>[3x]GAMAMSDLPIEFTELVDLMSLGISPQFLDFRSTTFESDHFVTVRETKDGTNSVAIVDLAKGNEVTRKNMGGDSAIMHPSQMVISVRANGTIVQIFNLETKSKLKSFTLDEPVIFWRWLSETTLGFVTARSILTSNVFDGNVNAKPQLLTLRHANLNNTQIINFVANKNLDWFAVVGILQENGRIAGRIQLFSKQRNISQAIDGHVAIFTNILLEGNGSTPVQVFVTGNRNATTGAGELRIIEIDHDASLPSQYQKETTDIFFPPDATNDFPIAVQVSEKYGIIYLLTKYGFIHLYELETGTNLFVNRITAESVFTAAPYNHENGIACINKKGQVLAVEISTSQIVPYILNKLSNVALALIVATRGGLPGADDL;>[9x]GVSLIDL

The protein that gives the process its name, Clathrin, is a triskelion composed of three heavy chains (Clathrin Heavy Chain, Chc) that provide the structural backbone of the lattice, further stabilized and regulated by three light chains (Clathrin Light Chain, Clc). The proximal domain specifically interacts with Clcs, whereas, the N-terminal domain (NTD) of Chc, which adopts a WD40 beta-propeller structure, is pivotal for interactions with various adaptor proteins (APs). To investigate the existence of binding sites present in Clathrin NTD, we crystallized the N-terminal domain of Chc with different peptides derived from adaptor proteins containing CBMs. All our structures show that each peptide binds to three different binding pockets (Clathrin, Arrestin and W-box).

Crystal structure of Chc-NTD (displayed as a grey cartoon) bound to CBMs from Ent1 (1.75 Å, red), Ent2 (1.74 Å, yellow), Ent5 (Ent5.1 LIDL motif, 2.01 Å, green), Apl2.1 (Apl2.1 LLDLF motif, 2.75 Å, blue) and Yap1801 (1.95 Å, grey). Zoom: individual Chc-NTD boxes with Ent2 CBM-containing peptide. For the Ent1 and Ent2 complexes, a water molecule bridges the interaction between the carbonyl oxygen at the motif’s +3 position and N64. Water-mediated interactions are also observed in the W-box between the NTD backbone (L24, D25 and V309) and the peptide at position +3, for both Ent1 and Ent2. Residue K284 within the W-box establishes salt bridges with the carboxy-terminal of Ent1, Ent2 and Yap1801. For the Chc-mScarlet/Ent2-mNeonGreen pair, mutation of the Arrestin box showed a significant decrease in FRET efficiency (9.02% for WT vs. 6.7% Arr), while the W and Cla mutants did not show significant changes. Ent2’s main target site appears to be the Arrestin box as shown in our FRET in vivo experiments. Mutation of the Clathrin box showed a reduction of almost seven-fold in the binding affinity to Ent1 (KDApp WT ≅ 138 µM vs. KDApp Cla ≅ 968 µM), while Ent2 exhibits a three-fold increase in its dissociation constant (KDApp Cla ≅ 509 µM). In the competitive landscape, Ent2 demonstrates reduced efficacy in counteracting Ent1’s occupancy, corroborating what was observed in the FRET experiments. Ent2 interactions are weaker, especially in the presence of Ent1 as a competitive binding partner.ALPHA,ALPHA,ALPHA-TRIFLUORO-P-CRESOL | C7 H5 F3 O | 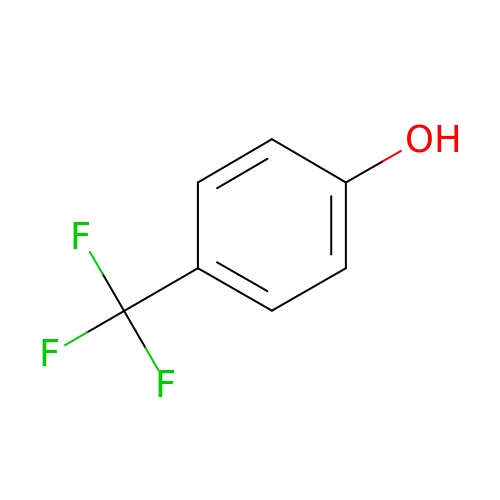BAYGVMXZJBFEMB-UHFFFAOYSA-N> YDPFKYVETVFVVDKAMVTKYNGDLDKIKTKMYEAANNMNEMYRYMFFRVVMVGLIIWTEEDKITVKPDVDYTLNAFAEWRKTYLLAEKKHDNAQLITGIDFRGSIIGYAYIGSM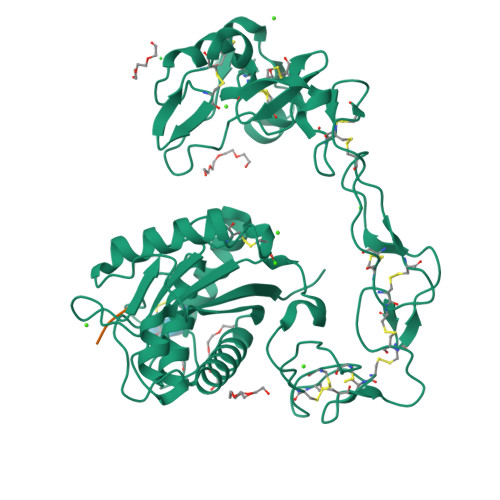CHPKRSVGIIQDYSPINLVLAVIMAHEMGHNLGIHHDDGYCYCGGYPCIMGPSISPEPSKFFSNCSYIQCWDFIMNHNPECIDNEPLGTDIISPPLCGNELLEVGEECDCGTPENCQNPCCDAATCKLKSGSQCGHGKCCEQCKFRTSGTECRASMSECDPAEHCTGQSSECPADVFHKNGEPCLDNYGYCYNGNCPIMYHQCYALFGADIYEAEDSCFESNKKGNYYGYCRKENGKKIPCASEDVKCGRLYCKDDSPGQNNPCKMFYSNDDEHKGMVLPGTKCADGKVCSNGHCVDVTTAY;> KNL>[12x]GSEFMDMEKRLRAEMQKAEDKA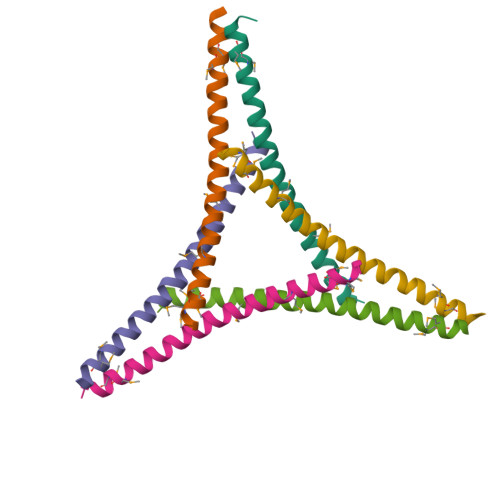VEHKEILDQLESLKLENRHLSEMVMKLELGLHEA5-methyl-N-[(pyridin-4-yl)methyl]pyridin-3-amine | C12 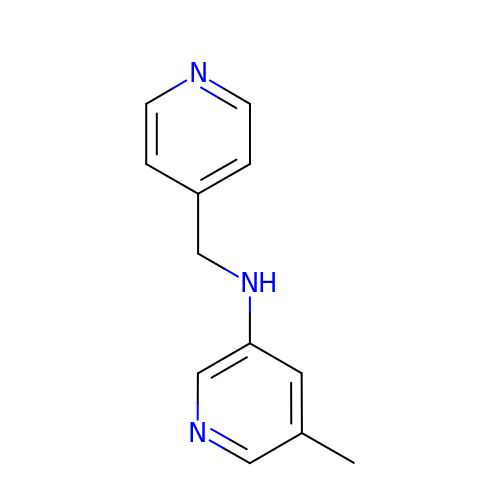H13 N3 | CKIRWILOFLBVIB-UHFFFAOYSA-N We have recently identified a periplasmic protein AztD in Paracoccus denitrificans, which is able to transfer zinc to the cluster A-I SBP AztC23. Here, we describe crystal structures of AztD homologs from P. denitrificans (PdAztD) and Citrobacter koseri (CkAztD), a pathogen of the carbapenem-resistant Enterobacteriacea group. In each case, the protein adopts a beta-propeller fold composed of continuous antiparallel beta sheets forming 8, 3-, and 4-stranded blades and containing a disulfide bond between highly conserved Cys214 and Cys231 (P. denitrificans numbering). Two high-affinity zinc-binding sites are identified, only one of which is competent for transfer to AztC.

The crystal structure of CkAztD was solved by single wavelength anomalous dispersion data collected on a crystal soaked with lead acetate. This structure was then used to solve the structures of native CkAztD and PdAztD using molecular replacement. The crystal structure of CkAztD has two monomers in the asymmetric unit while PdAztD has 4. All zinc occupancies refined to > 0.7 in PdAztD and 0.4 in CkAztD. Part of this variability likely arises from crystal-packing effects, particularly in the CkAztD structure. In the structure of native CkAztD, the feature containing site 2 in chain A projects into the pore of chain B, making a hybrid site with two zinc ions and His104 apparently bridging between them. A buffer molecule introduced during crystallization is also nearby in the pore. This suggested the possibility of associative, kinetically controlled transfer from site 1 to site 2 between two AztD molecules. Thus, if zinc is transferred associatively between AztD sites, this process does not compete with its dissociation to solution under these conditions, and the hybrid zinc site in the crystal structure of CkAztD is most likely an artifact of crystallization.

>[2x]MMENIMKKRLLSTSISTLLLGLSVMPAFADEDVTAWRLFIADHDKPVVNVIDALDGDKLATFNVKGPANLSRSESGATIFAIQGSAGVVSTIASGIAFHDHGDHADIDIDAPKLLPLELTGKKPGHFVERQGKIAQWFDGEDSAQILGESAVLKGQKNITKVNVVAPHHGVAVPYDNYAVVSIPNPDDASKRPVGARVVDLQGKKVGDDALCPGLHGSAGSGDTFALSCETGLLLITQKNAAPVIRHLPYAKTLPEGSTSTLIGGKGMQYFIGNYGPDRIILVDPTESDSFRLIQLPTRRVHFVVDPVRAKFAYVFTEDGKLNQIDVLKGEISQSVRVTDPYSMDGHWNDPRPRIAVADNKIYVTDPLKSKIIVLDATSFKKTSEISVEGQPFNIVAVGGSGKVHGEHHDHEAHHHDDHAH> GHHHHHHIEGRLGKFSQTCYNSAIQGSVLTSTCERTNGGYNTSSIDLNSVIENVDGSLKWQPSNFIETCRNTQLAGSSELAAECKTRAQQFVSTKINLDDHIANIDGTLKYELGKFSQTCYNSAIQGSVLTSTCERTNGGYNTSSIDLNSVIENVDGSLKWQPSNFIETCRNTQLAGSSELAAECKTRAQQFVSTKINLDDHI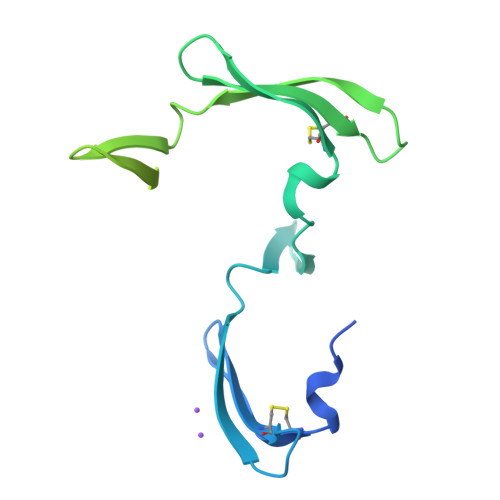ANIDGTLKYE>[2x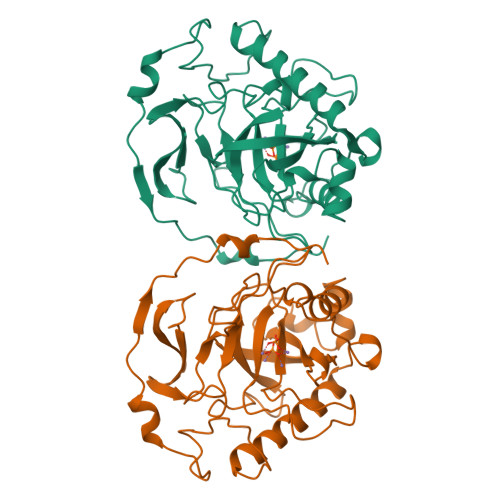]TYTTRQIGAKNTLEYKVYIEKDGKPVSAFHDIPLYADKENNIFNMVVEIPRWTNAKLEITKEETLNPIIQDTKKGKLRFVRNCFPHHGYIHNYGAFPQTWEDPNVSHPETKAVGDNDPIDVLEIGETIAYTGQVKQVKALGIMALLDEGETDWKVIAIDINDPLAPKLNDIEDVEKYFPGLLRATNEWFRIYKIPDGKPENQFAFSGEAKNKKYALDIIKETHDSWKQLIAGKSSDSKGIDLTNVTLPDTPTYSKAASDAIPPASLKADAPIDKSIDKWFFISGSV>STSPEIASLSWGQMKVKGSNTTYKDCKVWPGGSRTWDWRETGTEHSPGVQPADVKEVVEKGVQTLVIGRGMSEALKVPSSTVEYLK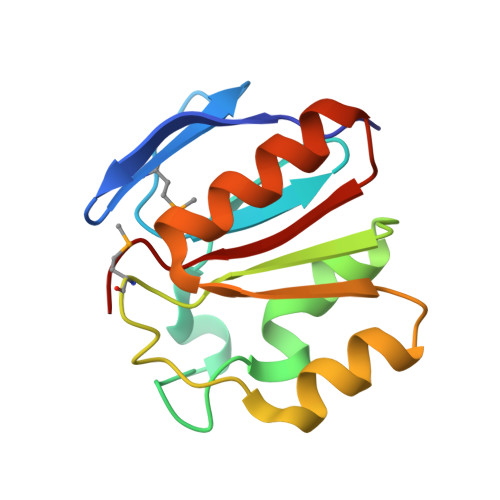KHGIDVRVLQTEQAVKEYNALVAQGVRVGGVFHSTC[2x]>SMSVA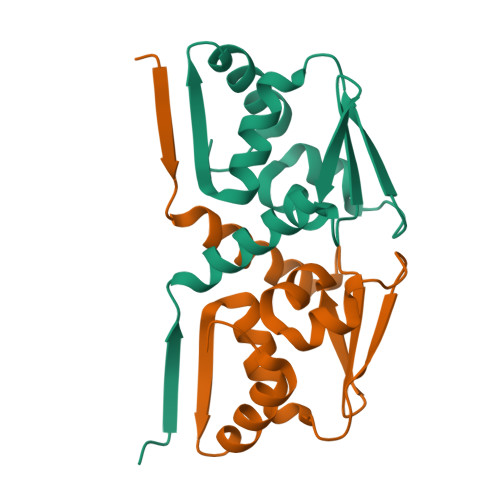AYESSVHSTNVLLSLNDQRKKDVLCDVTIFVEGQRFRAHRSVLAACSSYFHSRIVGQADGELNITLPEEVTVKGFEPLIQFAYTAKLILSKENVDEVCKCVEFLSVHNIEESCFQFLKF[2x]>MGSSHHHHHHHSSGLVPRGSHHMLEMQINLPEVHAEVTAQFVRYEKALTSNDTAVLNELFWNSPQTLRYGATENLYGYEAIAGFRATRSPNNLEREIVRTVITTYGHDFATANIEFRRLSHSQLTGRQSQTWMRTSQGWRVVAAHVSLIALPVS[4x]

AtzH is the first DUF3225 family protein that has been shown to possess a catabolic function, likely decarboxylating the product of AtzEG-mediated deamination of 1-carboxybiuret as part of the cyanuric acid mineralization pathway. The data presented here imply that AtzH is a decarboxylating, 1,3-dicarboxyurea amidohydrolase. AtzH belongs to NTF2-fold superfamily, which contains 38 protein families, including the AtzH family: DUF3225 (DUF: domain of unknown function). Size exclusion chromatography performed on AtzH after removal of the his-tag, suggested that the native protein had a molecular mass of ~ 29 kDa, consistent with a dimer (2 x 14,655 kDa).

We obtained the X-ray crystal structure of the AtzH. Differential Scanning Fluorimetry (DSF) was used to estimate the stability of the protein and showed that the native protein had a Tm of 57.2°C. Well diffracting crystals of AtzH grew readily, and two different space groups were observed: P1 and C2221. X-ray diffraction data were collected for both. Analysis with PISA gives an interfacial surface area of almost 3,200 Å2 (or about 29% of the total surface area of the protein). The AtzH active site was sought by examining the X-ray structure. However, an in silico docking simulation between the X-ray crystal structure of the AtzH dimer and 1,3-dicarboxyurea elucidated a potential active site. The arginine residues form an extensive hydrogen bonding network with the carbonyl oxygens of 1,3-dicarboxyurea. Tyr22 is positioned within 3 Å of the carbonyl carbon of one of the two terminal carboxylic acids, and Arg46 is within hydrogen-bonding distance of the hydroxyl group of Tyr22. Tyr22 and Arg46 are therefore well positioned to form a catalytic dyad, albeit one of atypical composition.2,2'-bipyridine | C10 H8 N2 | 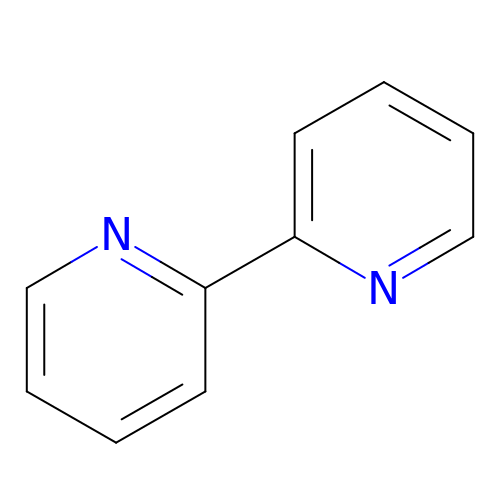ROFVEXUMMXZLPA-UHFFFAOYSA-N>MEQAPSEALQSLSVSDSQIPQSSNSTPQLSPEEKFKIVRSVGEECIQEDELLNLLTKKPEPVCYDGFEPSGRMHIAQGVMKTISVNKLTSAGCRVKIWIADWFAKLNNKMGGDLKKIETVGRYLIEIWKAVGMDVEGGKVEFLWSSKEINARADEYWPLVLDIAQKNNLKRIIRCSQIMGRSEQDELTAAQIFYPCMQCADIFFLKADICQLGMDQRKVNVLAREYCDDIKRKNKPIILSHHMLPGLQQGQEKMSKSDPSSSVFMEDEEAEVNVKIKKAYCPPKVVEGNPCLEYIKYLILPWFNEFTVERSADNGGNKTFKSYEELIADYESGELHPADLKPALSKSLNKILEPVREHFRKDSNAKELL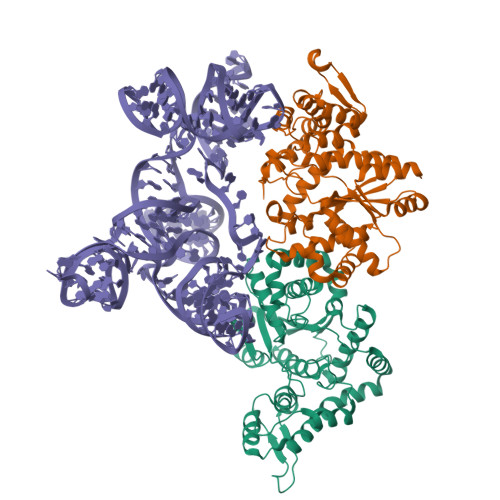KRVKAYRVTK[2x]> AVQVTFTVQKGSDPKKLVLDIKYTRPGDSLAEV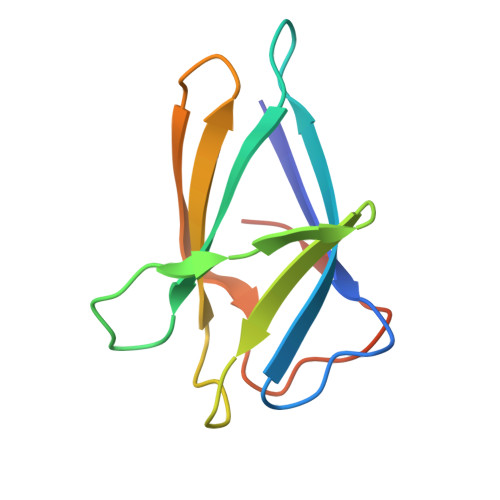ELRQHGSEEWEPLTKKGNVWEVKSSKPLVGPFNFRFMSKGGMRNVFDEVIPTAFSIGKTYKPEEQEF> MFLDTHKQLTLFTSEGKLDQCDNALKAATQGSLSVGCVSENGVVLASLKESNNLVILSEYKKIYQISPNLGITYSGCQPDFRIQYNLSLKISEEYTDIYSTNIPIRLFVEQFSRQIQEYTIKKGYRPFGTLLLIVGDNKMYRVDPSGSYTSLQVGTI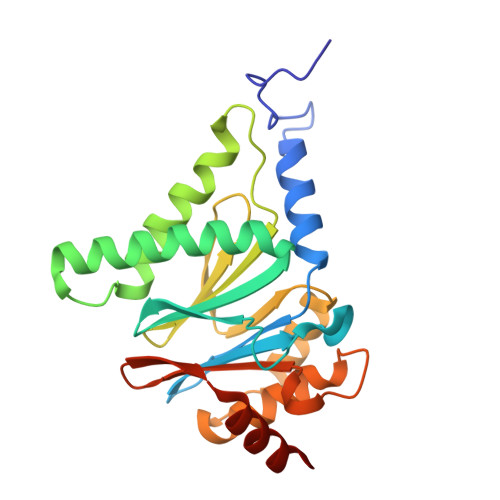GREYTESGRLLERRKGMLDDNISTCVECIREYCGRSVKSEDIDIGVYRGQEFRVYSKEEVQEVFDSINKI>GPLGSPNSEEEASVSVWDEEEDGATFTVTSRQYRPLDPLAPLPPPRSSRRLRAGTLEALVRHLLDARTAGADMMFTPALLATHRAFTSTPALFGLVADRLEALESYPPGELERTTGVAISVLSTWLASHPEDFGSEVKGQLDRLESFLLRTGYAAREGVVGGSADLIRNLRARVDPRAPDLPKPLALPGDSPADPTDVLVFLADHLAEQLTLLDAELFLNLIPSQCLGGLWGHRDRPGHSHLCPSVRATVTQFNKVAGAVVSSVLGATSIGEGPREVTVRPLRPPQRARLLEKWIRVAEECRLLRNFSSVYAVVSALQSSPIHRLRAAWGETTRDSLRVFSSLCQIFSEEDNYSQSRELLTQEVKPQPPVEPHSKKAPRSGFRGGGVVPYLGTFLKDLVMLDAASKDE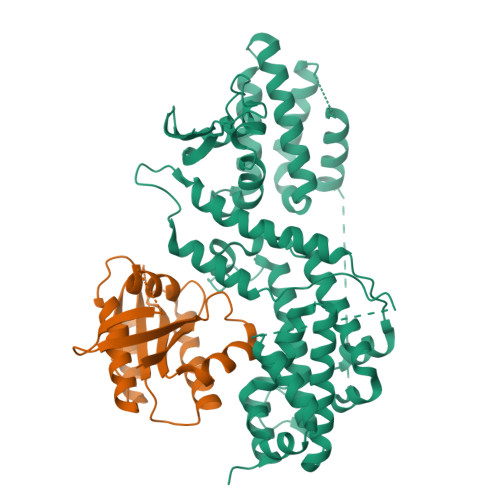LENGYINFDKRRKEFAILSELLRLQKECRGYDLRPNSDIQQWLQGLQPLTEAQSHRVSCEVEPPG[2x];>[2x]GSMSKKPTAGPALHKVIMVGSGGVGKSALTLQFMYDEFVEDYEPTKADSYRKKVVLDGEEVQIDILDTAGQEDYAAIRDNYFRSGEGFLCVFSITDDESFQATQEFREQILRVKNDESIPFLLVGNKCDLNDKRKVPLSECQLRAQQWAVPYVETSAKTRENVDKVFFDLMREIRSRKTEDSKATSGRAKDRCKKRRLKCTLL>MNLTDSLQNVLSGVGTLNRYRLDIPSCPSSLDVEDFSGTEGISKIYRYDIIFTSTDRYPDAAWFLRKSATLIMGTGLLESLTEQKKVHGVITDFRRISGSEDQAQYRITLKPFISLLDKQFRTHRFFVNKSVPEVVEQILTEHGLKGWEYEFSLKRTYPKREQINQYQESDLRFIQRLLAEVGIFYFFTLHPDAQTEVIHFGDVQAALIFDKTLPVNSPSGMSDSGTDSVWALNVEHRVVESRVITNDYNHREAQNILMSVPADMTRGEGYDTSYGEVYHYRPRHTERGDKIDPAPETANFWARLDHERFLAEQTRITGKSTDASLLPAQVLTITDSTPPVLPAPLQEPVLLTQLLFTGSRKSALQVMLSAVPYSEIVCWRPPLLTRPKITGTMTARVTSAKEGDIYAWQDASGMYRVKFDADRDDKNPGQESMPVRLAKPYSGDAYGFHFPLIQGTEVAIAFEEGDPDRPYIAHALHDSRHVDHVTDKNGTRNVIRTPANNKLRMEDKRGEEHIKLSTEYGGKTQLNLGHNVDASRELRGEGAELRTDDWISIRGGKGIFISADMQPQAQGKMLDMDEAIRQLEQALSLARSMAKAATAANATQGDISCQQRLNASLTDLTAPGMLLHAPDGIGMVSARALRIASGSESVGIMSGDNTDITAGQSFTVVAEGAVSLLSRNQGMQLLAAKGRVNIQAQSDDLSMSSQQNLDIQSSEGKVTVSANQELILACGGAYIKLSGGNIELGCPGQILLKSTNMQKMGPTSLDIASVEMPRGFGGGFILTDEAGVPQPSTPYRLTTAEGDILQGITDENGKTAPVNTSIPSVVKVEFGKVKIHGETE[3x];>MTKYQGYDVTDATHKTSIHNDWKVVVAKKKPARGVTLTIGIFFDGTGNNRENTASRLMKFNECSAARQGVNQKDAQSCEDFLKEINKNSISNGSYRGYYSNIHWLNILYHPDQVLKKDQTSAQIKTYISGIGTAAGEADSVIGMGLGTSILDIFEGVVTKTDEAMERITQALSEFMGFNLSPDFCIAKIQFDVFGFSRGAAAARHFANRVMEQDPAIARAIAKGLRGDFYDGKPSGEVRFLGLFDTVAAIGGISNFFDINGRSN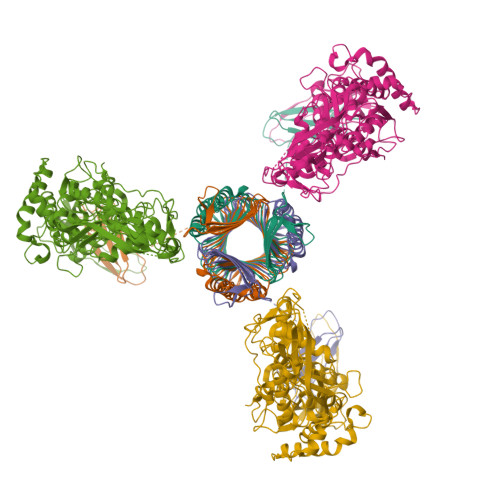PGVKLELRPSVAKKVFQITAMNEYRYNFSLNSIKGMWPELALPGAHSDIGGGYNPVGSPLQENESLFLSCPEFEIVSDDTREMDTRVYRKAEQVRKMLMTLPALKHILPHGKLTTKIRSIGVNNSNQRRAGVIQKQVGAAVFFERMAVPNDWANVCLRVMLDAAQEAGVLFEPIRQTNTELQLPSELIFLADKAIAQGKAVRLGQEPQAFTEEELYIIGKYTHCSANWNIESDGNLWVDPTTGEIFIHRFGPKGNKAFVFPNKPNDRWIRSVWYMDDQQRLNDNAVKNTKVMMSGV[3x]>GSAKDPMHNFTYWNPTKLIFGRGEVERLPEELKSYGKNVLLVYGGGSIKRSGLYDQVIEQLNKAGVTVHELAGVEPNPRVSTVNKGVALCKEHHIDFLLAVGGGSVIDCTKAIAAGAKYDGDAWDIVTKKHQPKDALPFGTVLTLAATGSEMNSGSVITNWETKEKYGWGSPLVFPKFSILDPVNTFTVPKNHTIYGMVDMMSHVFEQYFHHVSNTPYQDRMCESLLRTVIETAPKLINDLENYELRETILYTGTIALNGMLSMGARGDWATHNIEHAVSAVYDIPHAGGLAILFPNWMRHTLSENPARMKQLAVRVFGVEEAGKTDKEVALEGIDKLSAFWTSLGAPNRLADYDINDEQLDTIADKAMANGTFGQFKSLNKEDVLAILKAS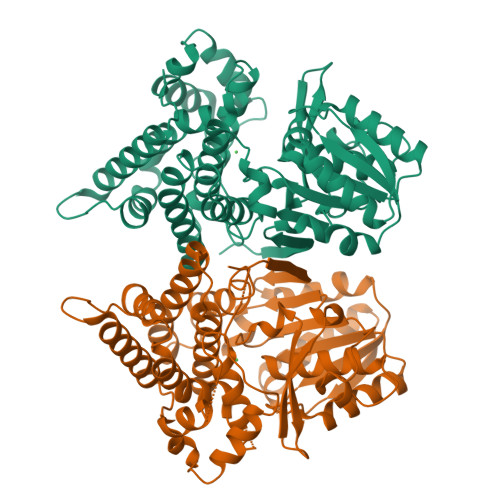L[2x]>HMALRVGIVYGTRPEAIKLAPLVLALDADPGFEPVIITTGQHRDMLDEINELFGLRPRHNLDIMRPGQRLSAMASRIVGELGDPLLDELVDVAVVQGDTSTAFAAAYAAACERIPVAHLEAGLRTGDRFEPFPEEINRRLITQLADLHFAPTADAAGNLLAEGVRSDDVYVTGNTVIDAMHLVLDRPGDSANRELDAFTEGRQTVLLTMHRRESWGIPMGRVAAAVAELCRSRPTLRFVIPLHPNPEVRRVFRSHL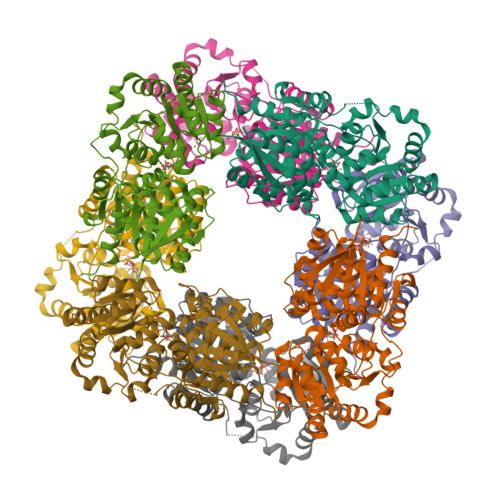SSLTQVLLCEPLRYSEFIRLMHRAVLVLTDSGGVQEEAPTLGKPVLVLRDRTERPEGIAAGCARLVGTDPALIVKEVGRLLDDPEAYEAMRRPGIVCYGEGDAAARCLEALRERWLSSP[8x]DESOXYCORTICOSTERONE 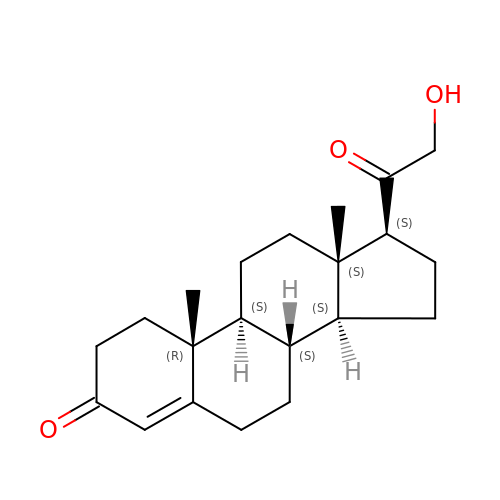| C21 H30 O3 | ZESRJSPZRDMNHY-YFWFAHHUSA-N1-[3-(2-methyl-4-thiophen-2-yl-1,3-thiazol-5-yl)propanoyl]piperidine-4-carboxamide 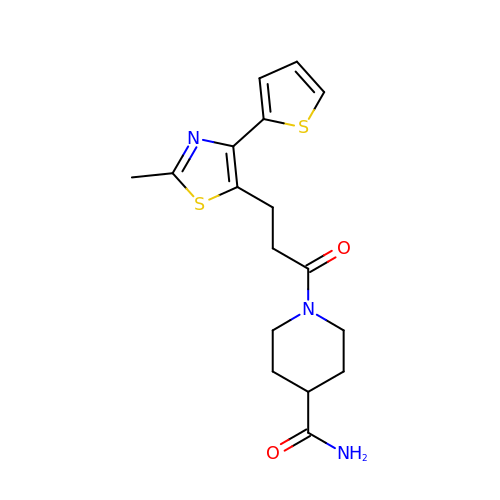| C17 H21 N3 O2 S2 | HRZYWKOZIFTEHZ-UHFFFAOYSA-N>[3x]PMFIVNTNVPRASVPDGFLSELTQQLA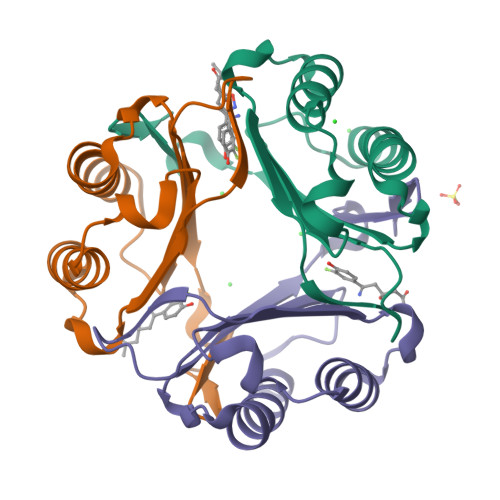QATGKPPQYIAVHVVPDQLMAFGGSSEPCALCSLHSIGKIGGAQNRSYSKLLCGLLAERLRISPDRVYINYYDMNAANVGWNNSTFA>SHAGANDLCQECEDIVHLLTKMTKEDAFQEAIRKFWEQECDILPWKLLWPRCRQVLDVYLPLWIDYFQSQIN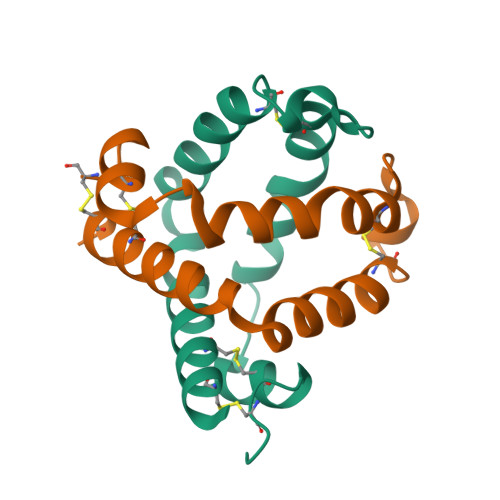PKAWCNHWGLCPRGQ[2x]2-fluoro-N-[4-(pyridin-4-yl)-1,3-thiazol-2-yl]benzamide 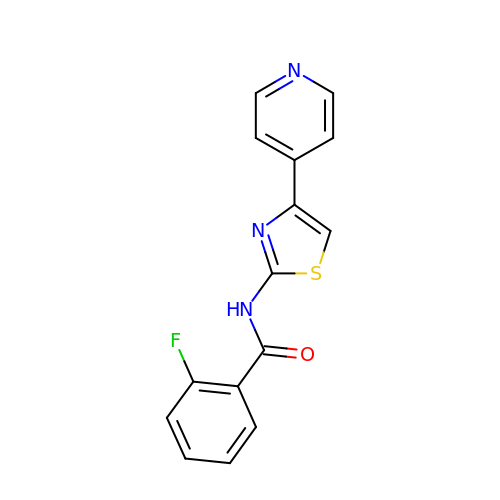| C15 H10 F N3 O S | OVEKVWJGWABLNU-UHFFFAOYSA-N>[2x]GSEDINRNPLLPTKEDEKMDGVIYGAYLPNLEKSVIPIGTASESTEPVNRYQIGVNLAGDAWAGYMSPRDNKFNGSKNFTNYFMYENWVNYVYSFMVTDVYSPWMQIKRISQ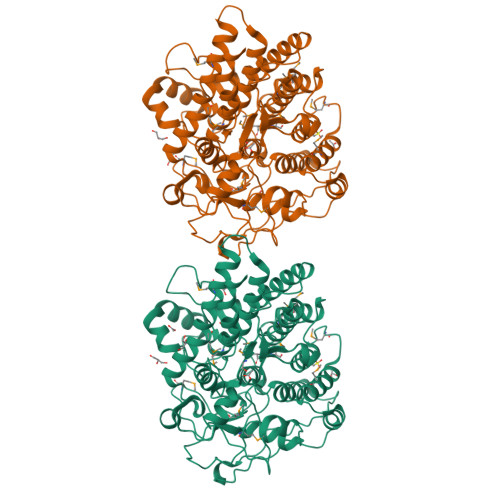DEGTRNDEIYALAQIIKIAALHRTTDMFGPIPYSQVGKGSFKVAYDSQESVYRSFLKELEEAVQTLDDYSNKSKEVLPAFDIVYNGDVNKWMRFANSLMLRLAIRVRFADAGLAKEYAEKAVKHPAGLINSKELAAQMGKGAGLQMKNPLKVINEEYNDTRMGATIYSYLAGYNDARAAVYFVKNNGFKAVRCGIAKSGDAYNGFTRPNVHEDDPLYWMKASEVCFLKAEGALAGFDMGGSAGDFYNAGIRMSFSENGLDNSSAETYLKDSTRKPANYTDTSNGELSANAPSSITIRWENGATEEEKLERIITQKYLAIFPNGQEAWTEWRRTGYPRQIVVAENKTNSAVLIGNGYDLGGVRRLPYPRTEYEQNGENLHNAISQYLGGVDNAATKVWWDKKSK>MGEVVRLTNSSTGGPVFVYVKDGKIIRMTPMDFDDAVDAPSWKIEARGKTFTPPRKTSIAPYTAGFKSMIYSDLRIPYPMKRKSFDPNGERNPQLRGAGLSKQDPWSDYERISWDEATDIVVAEINRIKHAYGPSAILSTPSSHHMWGNVGYRHSTYFRFMNMMGFTYADHNPDSWEGWHWGGMHMWGFSWRLGNPEQYDLLEDGLKHAEMIVFWSSDPETNSGIYAGFESNIRRQWLKDLGVDFVFIDPHMNHTARLVADKWFSPKIGTDHALSFAIAYTWLKEDSYDKEYVAANAHGFEEWADYVLGKTDGTPKTCEWAEEESGVPACEIRALARQWAKKNTYLAAGGLGGWGGACRASHGIEWARGMIALATMQGMGKPGSNMWSTTQGVPLDYEFYFPGYAEGGISGDCENSAAGFKFAWRMFDGKTTFPSPSNLNTSAGQHIPRLKIPECIMGGKFQWSGKGFAGGDISHQLHQYEYPAPGYSKIKMFWKYGGPHLGTMTATNRYAKMYTHDSLEFVVSQSIWFEGEVPFADIILPACTNFERWDISEFANCSGYIPDNYQLCNHRVISLQAKCIEPVGESMSDYEIYRLFAKKLNIEEMFSEGKDELAWCEQYFNATDMPKYMTWDEFFKKGYFVVPDNPNRKKTVALRWFAEGREKDTPDWGPRLNNQVCRKGLQTTTGKVEFIATSLKNFEEQGYIDEHRPSMHTYVPAWESQKHSPLAVKYPLGMLSPHPRFSMHTMGDGKNSYMNYIKDHRVEVDGYKYWIMRVNSIDAEARGIKNGDLIRAYNDRGSVILAAQVTECLQPGTVHSYESCAVYDPLGTAGKSADRGGCINILTPDRYISKYACGMANNTALVEIEKWDGDKYEIY[12x];>MEQYYMVIDVAKCQDCNNCFMGCMDEHELNEWPGYTASMQRGHRWMNIERRERGTYPRNDINYRPTPCMHCENAPCVAKGNGAVYQREDGIVLIDPEKAKGKKELLDTCPYGVMYWNEEENVAQKCTMCAHLLDDESWAPKMPRCAHNCGSFVYEFLKTTPEAMAKKVEEEGLEVIKPELGTKPRVYYKNLYRFEKNYVTAGILVQGDCFEGAKVVLKSGGKEVASA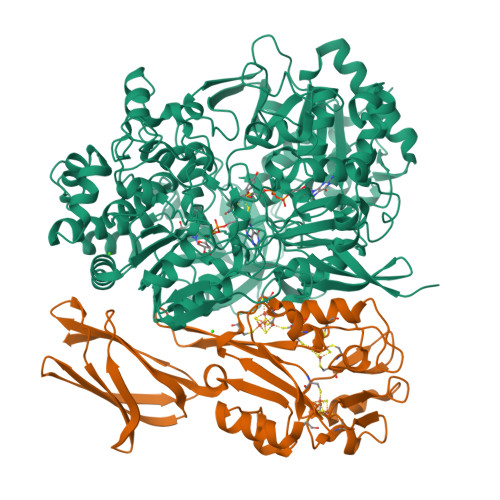ETNFFGEFKFDALDNGEYTVEIDADGKSYSDTVVIDDKSVDLGFIKL[12x]>ACMRVYITNINGQSIQSTAQLCQNTVTDVAVSLGYRELGIYCYQIHTDSESELSKRLDGIVAGLRHGDVVIFQTPTWNTTEFDEKLMNKLKLYDIKIVLFIHDVVPLMFSGNFYLMDRTIAYYNKADVVVAPSQKMIDKLRDFGMNVSKTVVQGMWDHPTQAPMFPAGLKREIHFPGNPERFSFVKEWKYDIPLKVYTWQNVELPQNVHKINYRPDEQLLMEMSQGGFGLVWMDDKDKEYQSLYCSYKLGSFLAAGIPVIVQEGIANQELIENNGLGWIVKDVEEAIM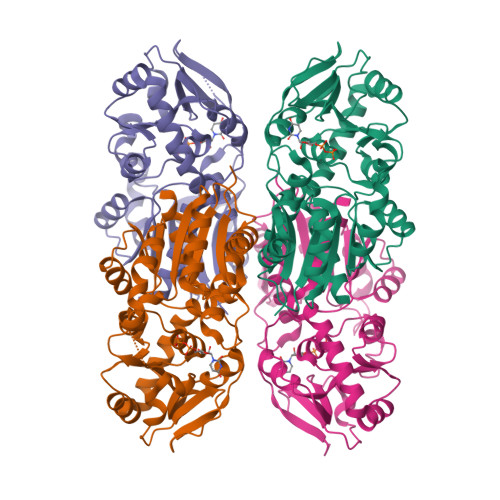KVKNVNEDEYIELVKNVRSFNPILRKGFFTRRLLTESVFQAICD[4x]>MDGVYVLSVKEDVPAAGILHAGDLITEIDGQSFKSSQEFIDYIHSKKVGDTVKIKYKHGNKNE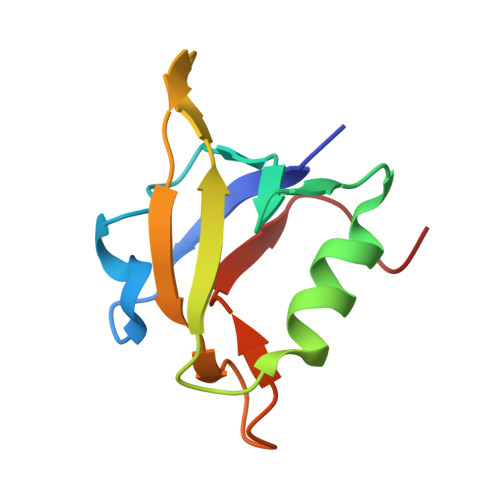EASIKLTAIDKKGTPGIGILEHHHHHH[2x]>[6x]MDSCHKIDYGLYALEILAQYHNVSVNPEEIKHRFDTDGTGLGLTSWLLAAKSLELKVKQVKKTIDRLNFISLPALVWREDGRHFILTKVSKEANRYLIFDLEQRNPRVLEQSEFEALYQGHIILIASRSSVTGKLAKFDFTWFIPAIIKYRKIFIETLVVSVFLQLFALITPLFFQVVMDKVLVHRGFSTLNVITVALSVVVVFEIILSGLRTYIFAHSTSRIDVELGAKLFRHLLALPISYFESRRVGDTVARVRELDQIRNFLTGQALTSVLDLLFSFIFFAVMWYYSPKLTLVILFSLPCYAAWSVFISPILRRRLDDKFSRNADNQSFLVESVTAINTIKAMAVSPQMTNIWDKQLAGYVAAGFKVTVLATIGQQGIQLIQKTVMIINLWLGAHLVISGDLSIGQLIAFNMLAGQIVAPVIRLAQIWQDFQQVGISVTRLGDVLNSPTESYHGKLALPEINGNITFRNIRFRYKPDSPVILDNINLSIKQGEVIGIVGRSGSGKSTLTKLIQRFYIPENGQVLIDGHDLALADPNWLRRQVGVVLQDNVLLNRSIIDNISLANPGMSVEKVIYAAKLAGAHDFISELREGYNTIVGEQGAGLSGGQRQRIAIARALVNNPKILIFDEATSALDYESEHIIMRNMHKICKGRTVIIIAHRLSTVKNADRIIVMEKGKIVEQGKHKELLSEPESLYSYLYQLQSD;>MKTWLMGFSEFLLRYKLVWSETWKIRKQLDTPVREKDENEFLPAHLELIETPVSRRPRLVAYFIMGFLVIAVILSVLGQVEIVATANGKLTLSGRSKEIKPIENSIVKEIIVKEGESVRKGDVLLKLTALGAEADTLKTQSSLLQTRLEQTRYQILSRSIELNKLPELKLPDEPYFQNVSEEEVLRLTSLIKEQFSTWQNQKYQKELNLDKKRAERLTILARINRYENLSRVEKSRLDDFDDTLEVTALVQNKDIGFINVGQNAIIKVEAFPYTRYGYLVGKVKNINLDAIEDQKLGLVF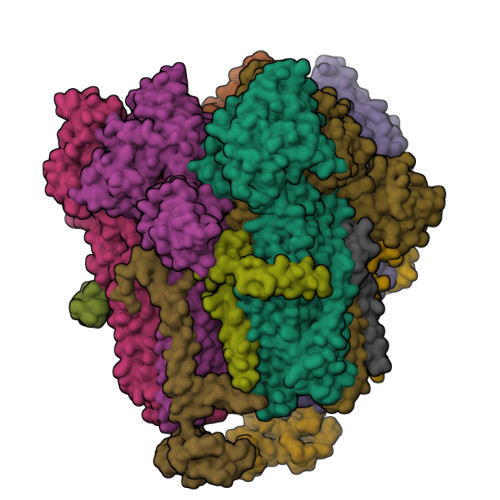NVIVSVEENDLSTGNKHIPLSSGMAVTAEIKTGMRSVISYLLSPLEESVTESLHER[6x]>[2x]TAELKICRVNRNSGSCLGGDEIFLLCDKVQKEDIEVYFTGPGWEARGSFSQADVHRQVAIVFRTPPYADPSLQAPVRVSMQLRRPSDRELSEPMEFQYLPDTDDRHRIEEKRKRTYETFKSIMKKSPFNGPTEPRP;> VFGYVTEDGDTALHLAVIHQHEPFLDFLLGFSAGHEYLDL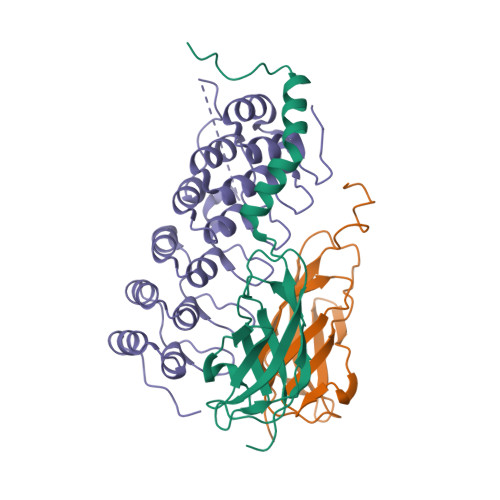QNDLGQTALHLAAILGEASTVEKLYAAGAGVLVAERGGHTALHLACRVRAHTCACVLLQPRPSHPRDASDTYLTQSQDCTPDTSHAPAAVDSQPNPENEEEPRDEDWRLQLEAENYDGHTPLHVAVIHKDAEMVRLLRDAGADLNKPEPTCGRTPLHLAVEAQAASVLELLLKAGADPTARMYGGRTPLGSALLRPNPILARLLRAHGAPEPEDGGDKLSPCSSSGSDSDSDNRDEGDEYDD>MSLTLDVWQHIRQEAKELAENEPMLASFFHSTILKHQNLGGALSYLLANKLANPIMPAISLREIIEEAYQS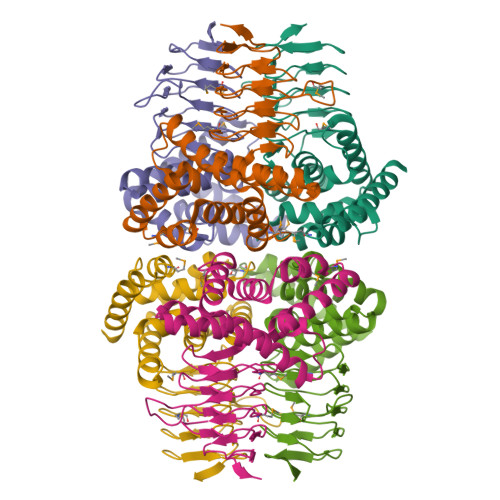NPSIIDCAACDIQAVRHRDPAVELWSTPLLYLKGFHAIQSYRITHYLWNQNRKSLALYLQNQISVAFDVDIHPAAKIGHGIMFDHATGIVVGETSVIENDVSILQGVTLGGTGKESGDRHPKVREGVMIGAGAKILGNIEVGKYAKIGANSVVLNPVPEYATAAGVPARIVSQDKAAKPAFDMNQYFIGIDDGMNLNEGGSHHHHHH[6x]> MAISRELVDPNSSPREIEVSEPREVGITELVLRDAHQSLMATRMAMEDMVGACADIDAAGYWSVECWGGATYDSCIRFLNEDPWERLRTFRKLMPNSRLQMLLRGQNLLGYRHYNDEVVDRFVDKSAENGMDVFRVFDAMNDPRNMAHAMAAVKKAGKHAQGTICYTISPVHTVEGYVKLAGQLLDMGADSIALKDMAALLKPQPAYDIIKAIKDTYGQKTQINLHCHSTTGVTEVSLMKAIEAGVDVVDTAISSMSLGPGHNPTESVAEMLEGTGYTTNLDYDRLHKIRDHFKAIRPKYKKFESKTLVDTSIFKSQIPGGMLSNMESQLRAQGAEDKMDEVMAEVPRVRKAAGFPPLVTPSSQIVGTQAVFNVMMGEYKRMTGEFADIMLGYYGASPADRDPKVVKLAEEQSGKKPITQRPADLLPPEWEKQ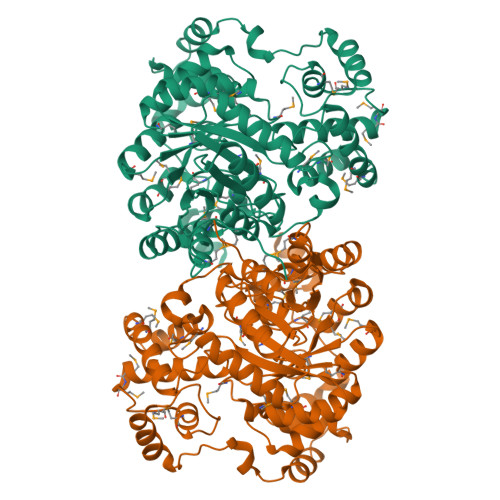SKEAATLKGFNGTDEDVLTYALFPQVAPVFFEHRAEGPHSVALTDAQLKAEAEGDEKSLAVAGPVTYNVNVGGTVREVTVQQATRASQPELAPEDPEDLEHHHHHH> SRSESSIENFLCRAACVYYATYTNNSEKGYAEWVINTRQVAQLRRKLELFTYLRFDLELTFVITSAQQPSTATSVDAPVQTHQIMYVPPGGPVPTKVTDYAWQTSTNPSVFWTEGNAPPRMSIPFISIGNAYSCFYDGWTQFSRNGVYGINTLNNMGTLYMRHVNEAGQGPIKS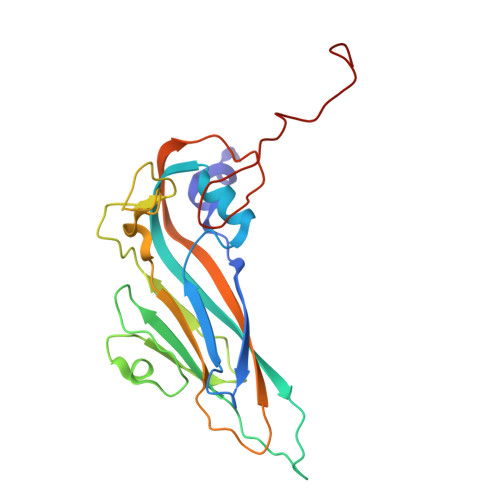TVRIYFKPKHVKAWVPRPPRLCQYEKQKNVNFTPTGVTTTRVGITT>[2x]MKIGVFDSGVGGFSVLKSLLKARLFDEIIYYGDSARVPYGTKDPTTIKQFGLEALDFFKPHEIELLIVACNTASALALEEMQKYSKIPIVGVIEPSILAIKRQVEDKNAPILVLGTKATIQSNAYDNALKQQGYLNISHLATS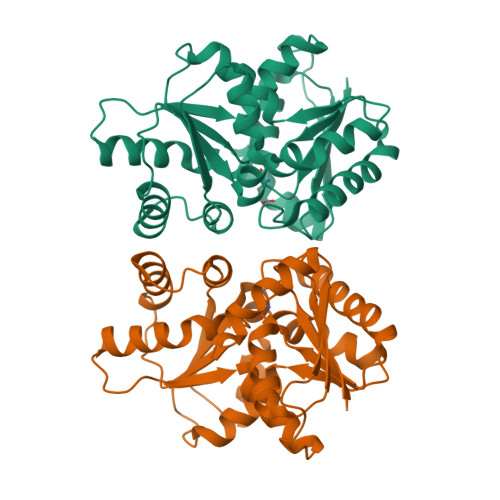LFVPLIEESILEGELLETCMHYYFTPLEILPEVIILGCTHFPLIAQKIEGYFMGHFALPTPPLLIHSGDAIVEYLQQKYALKNNACTFPKVEFHASGDVIWLERQAKEWLKL>[16x]MSRDRFRSRGGGGGGFHRRGGGGGRGGLHDFRSPPPGMGLNQNRGPMGPGPGGPKPPIPPPPPHQQQPQQPPPQQPPPQQPPPHQQPPPHQPPHQQPPPPPQDSSKPVVPQGPGSAPGVSPAPPPAGSAPPANPPTTGAPPGPGPTPTPPPAVTSATPGPPPPSTPSSGVSTTPPQSGGPPPPPAGGAGPGPKQGPGPGPGGPKGGKMPGGP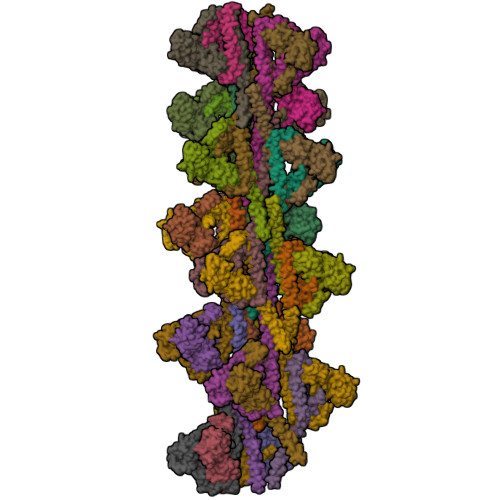KPGGGPGMGAPGGHPKPPHRGGGEPRGGRQHHPPYHQQHHQGPPPGGPAARTEEKISDSEGFKANLSLLRRPGEKTYTQRCRLFVGNLPADITEDEFKRLFAKYGEPGEVFINKGKGFGFIKLESRALAEIAKAELDDTPMRGRQLRVRFATHAAALSVRNLSPYVSNELLEEAFSQFGPIERAVVIVDDRGRSTGKGIVEFASKPAARKAFERCSEGVFLLTTTPRPVIVEPLEQLDDEDGLPEKLAQKNPMYQKERETPPRFAQHGTFEYEYSQRWKSLDEMEKQQREQVEKNMKDAKDKLESEMEDAYHEHQANLLRQDLMRRQEELRRMEELHSQEMQKRKEMQLRQEEERRRREEEMMIRQREMEEQMRRQREESYSRMGYMDPRERDMRMGGGGTMNMGDPYGSGGQKFPPLGGGGGIGYEANPGVPPATMSGSMMGSDMRTERFGQGGAGPVGGQGPRGMGPGTPAGYGRGREEYEGPNKKPRF;>[16x]MQSNKTFNLEKQNHTPRKHHQHHHQQHHQQQQQQQQQPPPPIPANGQQASSQNEGLTIDLKNFRKPGEKTFTQRSRLFVGNLPPDITEEEMRKLFEKYGKAGEVFIHKDKGFGFIRLETRTLAEIAKVELDNMPLRGKQLRVRFACHSASLTVRNLPQYVSNELLEEAFSVFGQVERAVVIVDDRGRPSGKGIVEFSGKPAARKALDRCSEGSFLLTTFPRPVTVEPMDQLDDEEGLPEKLVIKNQQFHKEREQPPRFAQPGSFEYEYAMRWKALIEMEKQQQDQVDRNIKEAREKLEMEMEAARHEHQVMLMRQDLMRRQEELRRMEELHNQEVQKRKQLELRQEEERRRREEEMRRQQEEMMRRQQEGFKGTFPDAREQEIRMGQMAMGGAMGINNRGAMPPAPVPTGTPAPPGPATMMPDGTLGLTPPTTERFGQAATMEGIGAIGGTPPAFNRPAPGADFAPNKRRRY> MDRKTRLSEPPTLALRLKPYKTAIQQLRSVIRALKENTTVTFLPTPSLILQTVRSHCVSKITFNSSCLYITDKSFQPKTINNSTPLLGNFMYLTSSKDLTKFYVQDISDLSAKISMCAPDFNMEFSSACVHGQDIVRESENSAVHVDLDFGVVADLLKWIGPHTRVKRNVKKAPCPTGTVQILVHAGPPAIKFILTNGSELEFTSNNRVSFHGVKNMRINVQLKNFYQTLLNCAVTKLPCTLRIVTEHDTLLYVASRNGLFAVENFLTEEP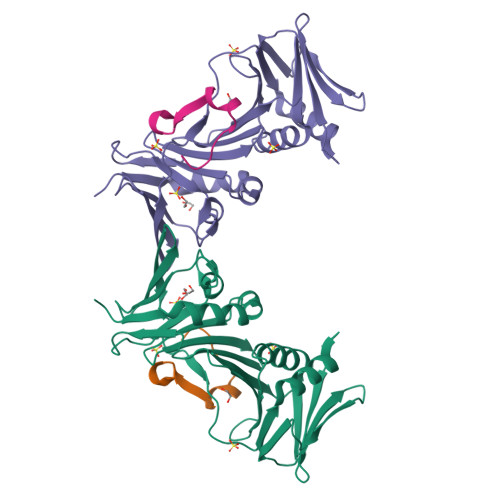FQRGDPFDKNYVGNSGKSR;> LPRRLHLEPAFLPYSVKAHECC> LPTRTATFERIPLKKMPSVREILEERGVDMTRLSAEWGVFTKRPSLTNLTSPVVLTNYLNTQYYGEIGIGTPPQTFKVIFDTGSANLWVPSTKCSRLYLACGIHSLYESSDSSSYMENGSDFTIHYGSGRVKGFLSQDSVTVGGITVTQTFGEVTELPLIPFMLAKFDGVLGMGFPAQAVGGVTPVFDHILSQGVLKEEVFSVYYNRGSHLLGGEVVLGGSDPQHYQGNFHYVSISKTDSWQITMKGVSVGS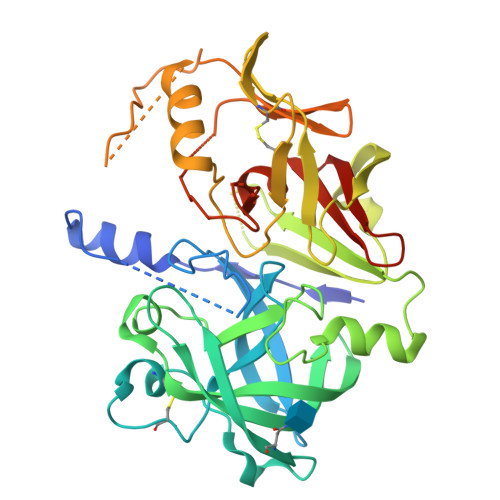STLLCEEGCAVVVDTGSSFISAPTSSLKLIMQALGAKEKRIEEYVVNCSQVPTLPDISFDLGGRAYTLSSTDYVLQYPNRRDKLCTLALHAMDIPPPTGPVWVLGATFIRKFYTEFDRHNNRIGFALARAAHHHHHH> GSA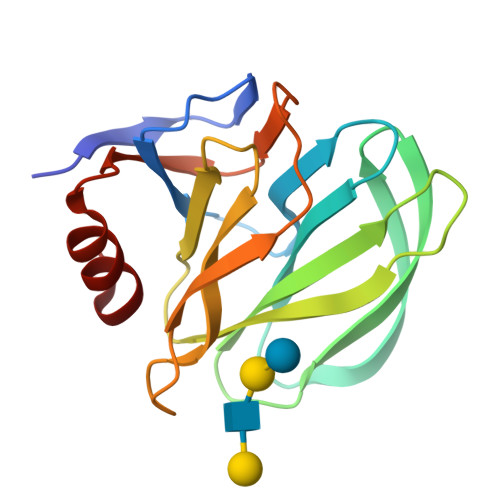LDGPYTPDSSNLPSNYWYLINPLNDGVVFSVTNNSTFWMFTYLILPNTAQTNVTVNVMNETVNISIDNSGSTYRFVDYFKTSSTQSYRQRNYLITEHRLQAYRRDESGNISNYWGSSTYGDLRVGTYFNPVLNAVINLNADFYIIPDSQQEKCTEYIKGGL> MSVLTKAIVNADAEARYLSPGELDRIKSFVASGERRLRIAQTLTEARERIVKQAGDQLFQIRPDVVSPGGNAYGEKMTALCLRDLDYYLRLVTYGIVAGDVTPIEEIGIIGVKEMYNSLQTPIPAVAEGVRAMKNVATSLLSGDDAAEAGFYFDYLVGAMQ;> MQDAITAVINNYDVQGKYLDGAALDKLKAYFTT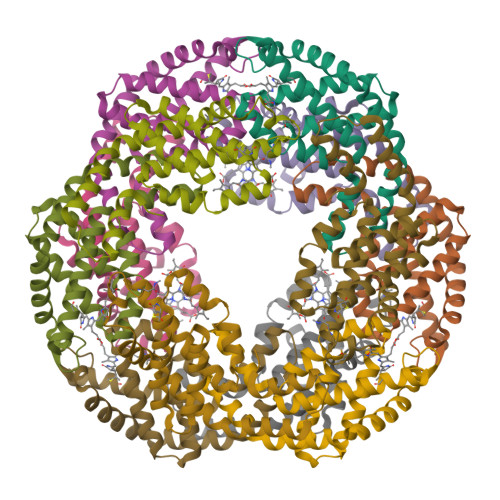GAVRVRAAAVISSNATTIIKEAAAKALIYSDLTRPGGNMYTTRRYAACIRDMDYFLRYATYAMLAGDPSILDERVLNGLKETYNSLGVPIAATVGGIQAMKEVVGGLVGPDAAKEASIYFDYLSSGLS Vinculin is composed of a N-terminal globular head domain, which consists of 4 α-helical bundles (D1-D4), that are connected to a C-terminal tail via a flexible hinge. The structures show that all vinculin variants consist of five helix-bundle domains four of which (D1-D4) form the vinculin head (Vh) that is connected through a long, partially unresolved, linker (“hinge”) to the fifth helical bundle (tail domain; Vt). In the closed conformer, Vt appears as a rod whose two ends bind to head domains D1 and D4, via residues conserved in vinculin and metavinculin; a small additional contact is made with D3.

In addition to comparing the energy required to open vinculin to that of vinculin-T12, we have created a novel variant of T12 termed T12-A974K, which contains an additional positive charge that might further destabilize head-to-tail interactions, leading to facilitated activation. Surprisingly, comparison of the new T12-A974K structure with the published structure of WT vinculin and of mVin indicated that despite the loss of 4 hydrogen bonds and the weakening of the remaining ones, the crystal structure clearly displayed a closed conformation. The T12 and T12-A974K mutation sites (residues D974, K975, R976 and R978) map to the Vt-D4 interface and hit hydrogen bonds that stabilize this interface (T974-N773, K975-E772 and R978-E775). The loss of these hydrogen bonds also leads to lengthening of hydrogen bonds between back-bone atoms in T12-A974K. Anchor residues N773 and E775 form hydrogen bonds to the side chains of D974 and R978, respectively; mutation of these residues to alanine would significantly weaken the Vt-D4 interactions in vinculin-T12 and vinculin-T12-A974K compared to native vinculin. In T12-A974K the additional positive charge augments the positive potential on the Vt side of the Vt-D4 interface. The structure, however, shows that K974 does not form a hydrogen bond with D4; rather, hydrophobic contacts between the CH2 groups of K974 and the side chain of N773 are observed. The number of contacts involving K974 exceeds the number of contacts that A974 can make and together with the augmented positive potential it is possible that the Vt-D4 contact in vinculin-T12-A974K is stronger than in vinculin-T12. Interestingly, the C state of vinculin-T12-A974K persists longer than that of the T12 variant, but the SO state, detected at low voltage just like in T12, is considerably less stable, and occurs for only a narrow range of collision voltages, before the next transition to the O state takes place. Another interesting observation is that T12 expression in cells converts FAs to force independent, while T12-A974K exerts a nearly opposite effect - namely its destabilization of FA in Y27632 cells.

> MPVFHTRTIESILEPVAQQISHLVIMHEEGEVDGKAIPDLTAPVAAVQAAVSNLVRVGKETVQTTEDQILKRDMPPAFIKVENACTKLVQAAQMLQSDPYSVPARDYLIDGSRGILSGTSDLLLTFDEAEVRKIIRVCKGILEYLTVAEVVETMEDLVTYTKNLGPGMTKMAKMIDERQQELTHQEHRVMLVNSMNTVKELLPVLISAMKIFVTTKNSKNQGIEEALKNRNFTVEKMSAEINEIIRVLQLTSWDEDAWASKDTEAMKRALASIDSKLNQAKGWLRDPSASPGDAGEQAIRQILDEAGKVGELCAGKERREILGTCKMLGQMTDQVADLRARGQGSSPVAMQKAQQVSQGLDVLTAKVENAARKLEAMTNSKQSIAKKIDAAQNWLADPNGGPEGEEQIRGALAEARKIAELCDDPKERDDILRSLGEISALTSKLADLRRQGKGDSPEARALAKQVATALQNLQTKTNRAVANSRPAKAAVHLEGKIEQAQRWIDNPTVDDRGVGQAAIRGLVAEGHRLANVMMGPYRQDLLAKCDRVDQLTAQLADLAARGEGESPQARALASQLQDSLKDLKARMQEAMTQEVSDVFSDTTTPIKLLAVAATAPPDAPNREEVFDERAANFENHSGKLGATAEKAAAVGTANKSTVEGIQASVKTARELTPQVVSAARILLRNPGNQAAYEHFETMKNQWIDNVEKMTGLVDEAIDTKSLLDASEEAIKKDLDKCKVAMANIQPQMLVAGATSIARRANRILLVAKREVENSEDPKFREAVKAASDELSKTISPMVMDAKAVAGNISDPGLQKSFLDSGYRILGAVAKVREAFQPQEPDFPPPPPDLEQLRLTDELAPPKPPLPEGEVPPPRPPPPEEKDEEFPEQKAGEVINQPMMMAARQLHDEARKWSSKGNDIIAAAKRMALLMAEMSRLVRGGSGTKRALIQCAKDIAKASDEVTRLAKEVAKQCTKAAIATNLLQVCERIPTISTQLKILSTVKATMLGRTNISDEESEQATEMLVHNAQNLMQSVKETVREAEAASIKIRTDAGFTLRWVRKTPWYQ>MMVIDTSALVAMLSDEPDAERFEAAVEADHIRLMSTASYLETALVIEARFGEPGGRELDLWLHRAAVDLVAVHADQADAARAAYRTYGKGRHRAGLNYGDCFSYGLAKISGQPLLFKGEDFQHTDIATVALP[4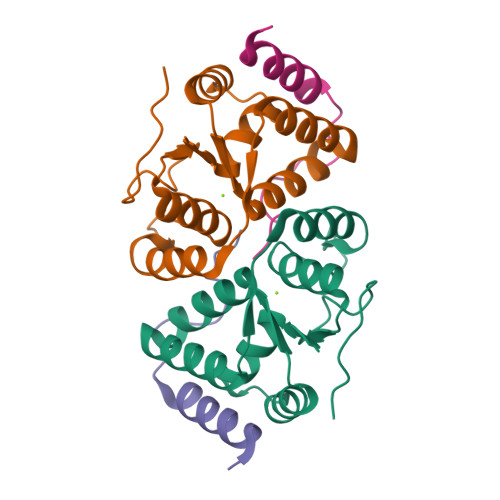x];>MALSIKHPEADRLARALAARTGETLTEAVVTALRERLARETGRARVVPLRDELAAIRHRCAALPVVDNRSAEAILGYDERGLPA[4x]> QHNPNTRDGRTAIVHLFEWRWADIAAECERFLGPKGFAGVQISPPNEHILVSSPWRPWWQRYQPISYNLCSRSGGENELRDMITRCNNVGVNVYVDAVINHMCGAGGGEGTHSSCGSWFNANNKDFPSVPYSNLDFNDGKCKTGSGNIENYGDPYQVRDCRLVGLLDLALEKDYVRGKVADFMNKLIDMGVAGFRVDACKHMWPGDLDNVYRRLNNLNTKWFPGGSRPFIFQEVIDLGGEPITTGEYVGLGRVTEFKYGARLGELFRKWNGQKLSYTKNWGEGWGFMADGNAVVFTDNHDNQRGHGAGGASILTFWDPRLYKMAVGYMLAHPYGFTRVMSSYSWDRNF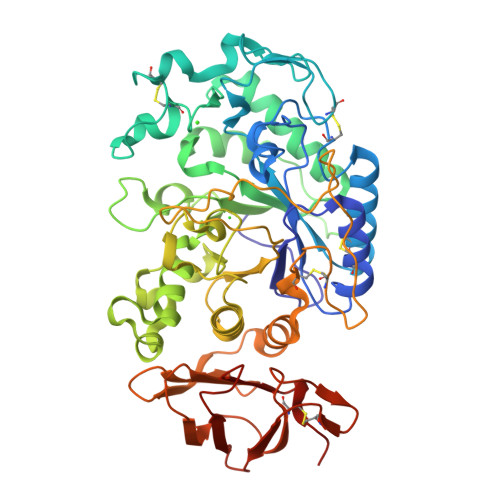VNGKDENDWIGPPSNGDGSTKPVPINPDQTCGDGWVCEHRWRQIMNMVQFRNVVNGQPHANWWDNGNNQVAFGRGNRGFIVFNNDDWALDVTLNTGLPGGTYCDVISGNKDGGSCTGKQITVGGDGRAHFYINNSEEDPFIAIHADSKLHHHHHHHH> GAGCAGACGTGACCGCACTCA;> GGTCA;> TCTGAGTGC;> 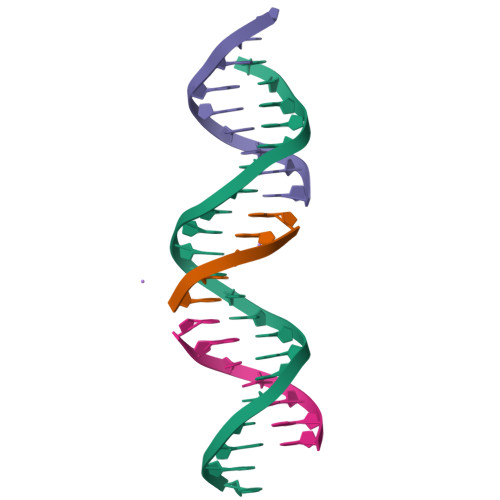CGTCTGC> MAELEKTFALIKPDAVRAGKAQEIMQLIELNGFTIIAKQKLQLTRARAEEFYGEHKGKEFFPKLVNFMTSGPIWALVLAKPGAILAWRALMGPTNVFKARAEQPKCLRALYGTDGTQNATHGSDSPISAAREIKFFFPTLSGDPTIYAEPTAAAEYITKRIQPALAKALAALAREKPSADKFEAITFVAGYLLQNNPNKPKVLMPDEWDPALMGDDEDDEADFINARLAAPTGNDGATKAEFDAMVEAAKADTGGAAPAQEFVYPDSKPTTPVVPAPPAPGSKPPSASGARPQSARPTSARPPSASAAPPAPLAPVPPPASSSRPASGSGRPPSATARPPSATPPPPPPAVELEEADDPAQLDEAATKVQAAFRGYQARKEVAVMRSEAQPGEAAAEPEQEAELQPEAEPEPQPEGEQEPQPQASASSSFLPDGVTEEMAAEAATRVQAHMRGHLARK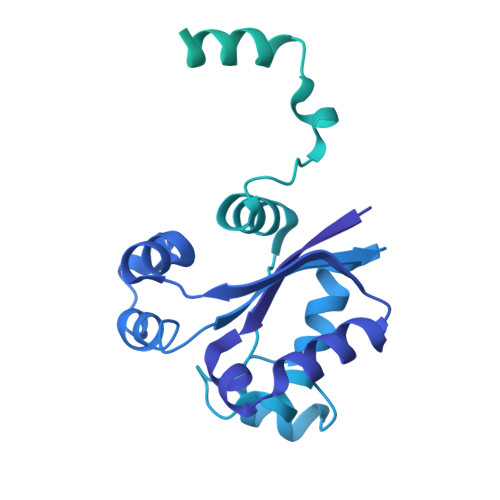QVAAIKAQQAAPAVAESSEALAEPEPQPEAEAEPQPQASVSSSFLPDGVTEEMAAEAATLVQAHMRGHLARKQVAAIKAQQAAPAVAESSEAQAEAEQTEAEAEPQPDAEAEAGAAEGEAEPEPEAAE>GAMASSKLNEDISLIEKQTSGRIGVSVWDTQTDERWDYRGDERFPLMSTFKTLACATMLSDMDSGKLNKNATARIDERNIVVWSPVMDKLAGQSTRIEHACEAAMLMSDNTAANLVLNEIGGPKAVTLFLRSIGDKATRLDRLEPR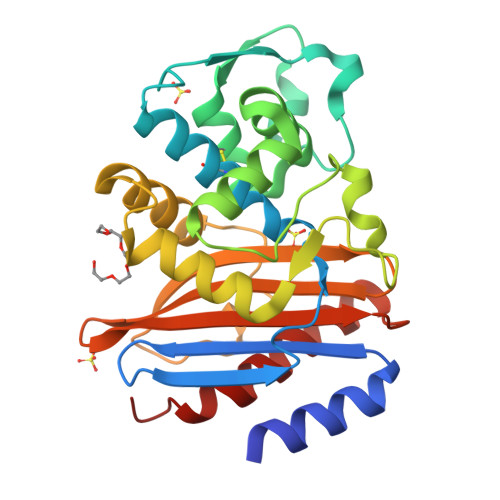LNEAKPGDKRDTTTPNAMVNTLHTLMEDNALSYESRTQLKIWMQDNKVSDSLMRSVLPKGWSIADRSGAGNYGSRGISAMIWKDNYKPVYISIYVTDTDLSLQARDQLIAQISQLILEHYKES[2x]CORTISTATIN A | C30 H36 N2 O3 | 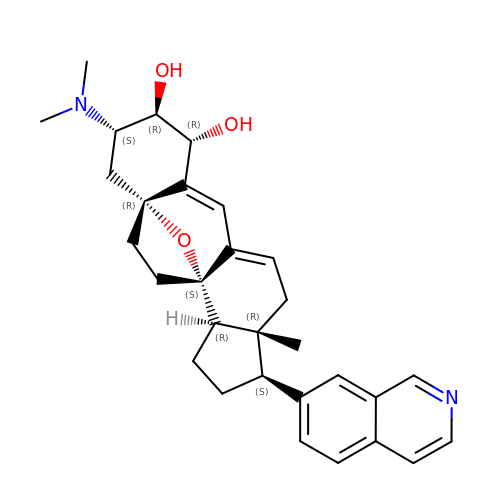KSGZCKSNTAJOJS-DZBMUNJRSA-N MtbTOP1 and topoisomerase I present in all bacterial pathogens are type IA topoisomerases that are needed for resolving topological barriers that require the passage of DNA through the break created on single-stranded DNA (ssDNA). M. tuberculosis topoisomerase I (MtbTOP1) is a validated target for much needed new antibiotics that can be used against the MDR-TB (multidrug-resistant tuberculosis) cases that are difficult to treat (1–3). The MtbTOP1-704t construct includes four N-terminal domains (D1–D4) and one C-terminal domain (D5). D1–D4 form a toroidal assembly found in all topoisomerase IA while D5 represents the Topo_C_Rpt subgroup of bacterial topoisomerase C-terminal repeats.

Compared to the structure of MtbTOP1-704t/ssDNA in the absence of metal ion, the extra electron densities in an approximately globular shape between the scissile phosphate and the carboxyl groups of E24 and D111 strongly indicate a site of bound Mg2+ ion. One water molecule, W1, was assigned to coordinate the metal ion, forming a distorted octahedral geometry with one ligand missing. It should be mentioned that the position of the side chain of D111 is not well-defined in electron density maps, suggesting that this residue can adopt multiple positions, with one of the positions engaged in metal binding. Interestingly, the water W1 can form a hydrogen bond with another TOPRIM acidic residue, D113, proposed previously to interact with Mg2+. To evaluate any conformational change possibly induced by Mg2+ binding, two structures, MtbTOP1-704t/MTS2–11 and MtbTOP1-704t/MTS2-13/Mg were superimposed. The resulted small rmsd value of 0.69 Å from the alignment indicates no overall structural impact upon Mg2+ binding. A close examination of their active sites also found no major changes aside from the side chain of R344, which moved away >0.6 Å from Y342 and the scissile phosphate. Considering that the ssDNA is intact and that the distance between Y342 hydroxyl and the phosphorous of the scissile phosphate is 3.13 Å, we propose that this MtbTOP1-704t/MTS2-13/Mg structure may represent an enzyme-ssDNA complex following DNA religation in the presence of Mg2+, as further elaborated later. In the structure with MTS2-13 in the presence of Mg2+, E24 is critical in forming and positioning the binding site for Mg2+, which can then increase the nucleophilicity of the 3′-OH during DNA religation. The position of E24 in the MtbTOP1-704t/MTS2-13/Mg structure also supports the assignment of this structure as the likely structure following DNA religation.

> SNAADPKTKGRGSGGNGSGRRLVIVESPTKARKLASYLGSGYIVESSRGHIRDLPRAASDVPAKYKSQPWARLGVNVDADFEPLYIISPEKRSTVSELRGLLKDVDELYLATDGDREGEAIAWHLLETLKPRIPVKRMVFHEITEPAIRAAAEHPRDLDIDLVDAQETRRILDRLYGYEVSPVLWKKVAPKLSAGRVQSVATRIIVARERDRMAFRSAAYWDILAKLDASVSDPDAAPPTFSARLTAVAGRRVATGRDFDSLGTLRKGDEVIVLDEGSATALAAGLDGTQLTVASAEEKPYARRPYPPFMTSTLQQEASRKLRFSAERTMSIAQRLYENGYITYMRTDSTTLSESAINAARTQARQLYGDEYVAPAPRQYTRKVKNAQEAHEAIRPAGETFATPDAVRRELDGPNIDDFRLYELIWQRTVASQMADARGMTLSLRITGMSGHQEVVFSATGRTLTFPGFLKAYVETVDELVGGEADDAERRLPHLTPGQRLDIVELTPDGHATNPPARYTEASLVKALEELGIGRPSTYSSIIKTIQDRGYVHKKGSALVPSWVAFAVTGLLEQHFGRLVDYDFTAAMEDELDEIAAGNERRTNWLNNFYFGGDHGVPDSVARSGGLKKLVGINLEGIDAREVNSIKLFDDTHGRPIYVRVGKNGPYLERLVAGDTGEPTPQRANLSDSITPDELTLQVAEELFAT> GTRPNHTIYINNLNSKIKKDELKKSLHAIFSRFGQILDILVPRRRTPRGQAFVIFKEVSSATNALRSMQGFPF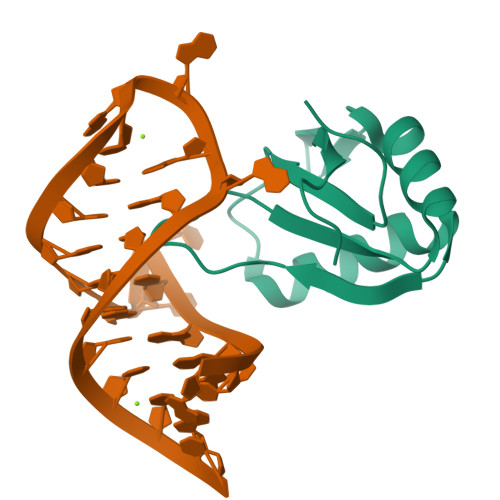YDKPMAIQYAKTDR Bromodomains (BRDs) are protein interaction modules that specifically recognize ε-N-lysine acetylation motifs, a key event in the reading process of epigenetic marks. The 61 BRDs in the human genome cluster into eight families based on structure/sequence similarity. Despite large sequence variations, all BRD modules share a conserved fold that comprises a left-handed bundle of four α helices (αZ, αA, αB, αC), linked by loop regions of variable length (ZA and BC loops), which line the Kac binding site and determine binding specificity. The four helices form a deep cavity that is extended by the two loop regions (ZA and BC loops), creating a largely hydrophobic Kac binding pocket.

Indeed, ITC experiments showed that the binding affinity of many BRDs was significantly increased for multiply modified peptides. For example, the KD of CREBBP decreased from 733 μM for H3K14ac to 131 μM for H3pS10K14acK18ac suggesting that many BRDs recognize a pattern of modifications rather than a single Kac mark. As a consequence, BRD acetyl-lysine binding sites are deep and largely hydrophobic binding pockets that represent attractive targeting sites for the development of Kac competitive inhibitors.

>SMRKKIFKPEELRQALMPTLEALYRQDPESLPFRQPVDPQLLGIPDYFDIVKNPMDLSTIKRKLDTGQYQEPWQYVDDVWLMFNNAWLYNRKTSRVYKFCSKLAEVFEQEIDPVMQSLG[2x]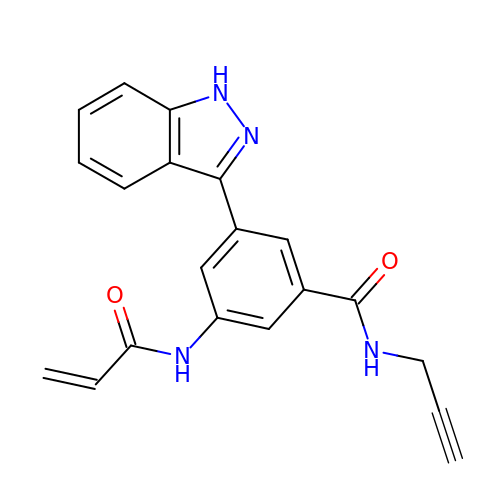3-(1H-indazol-3-yl)-5-(prop-2-enoylamino)-N-prop-2-ynyl-benzamide | C20 H16 N4 O2 | QLVGPPRZJNJOLD-UHFFFAOYSA-N>[2x]MELVSVAALAENRVI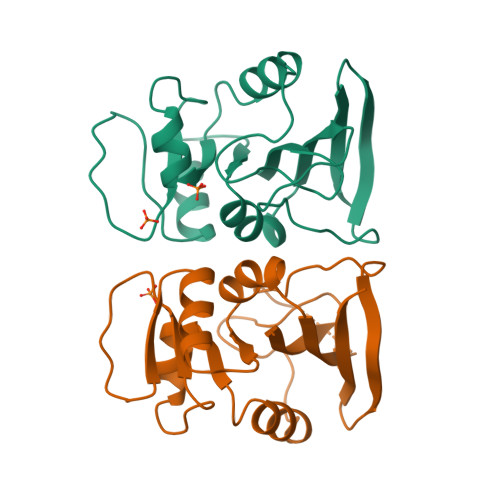GRDGELPWPSIPADKKQYRSRIADDPVVLGRTTFESMRDDLPGSAQIVMSRSERSFSVDTAHRAASVEEAVDIAASLDAETAYVIGGAAIYALFQPHLDRMVLSRVPGEYEGDTYYPEWDAAEWELDAETDHEGFTLQEWVRSASSR> RRSAWVFVAPWVPPPRHDVKVTMPPPPGGEVGGSYGVSTGYSDRLARTPYWKRMALSTYALRMKENET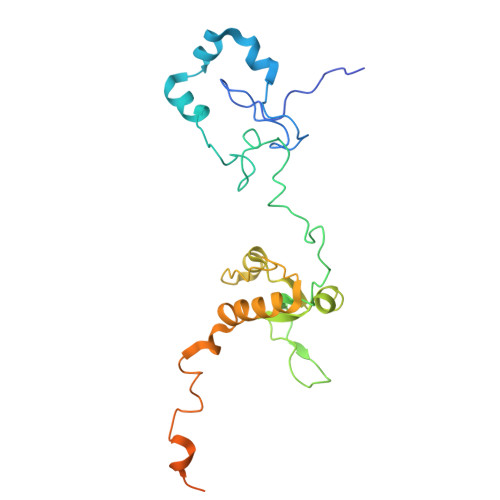RYPMSPHREGEYDLRYTVTAYPDHIKHRPLLEIGEAHQIPTIEIPVIFLVNLWDEERLTWFGRQYETVYVNRNVAREELLPQRYAIYATEEAYKLLGLPVVNHSIHEEIPKTPHAYKKLLEKQSYTEERWKYTIEYLFRKYEADPPELQDKSEDGWDGVEELATSATAGGAGDSLAKRKGPVKQRKARKIKLF cyclopropyl-[5-[[4-[4-[[(3~{S},4~{S})-3-methoxy-4-oxidanyl-pyrrolidin-1-yl]methyl]-3-methyl-pyrazol-1-yl]pyrimidin-2-yl]amino]-1-methyl-indol-3-yl]methanone | C27 H31 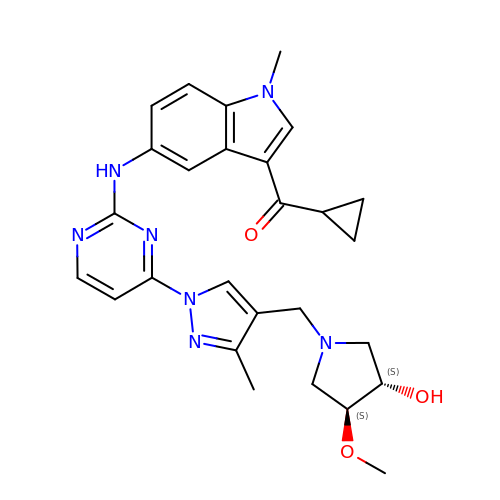N7 O3 | CBNDBWHBUUWRCT-ZEQRLZLVSA-N> MRTYSSLLEEFATELGLEEIETNELGHGAVTIDKIWVVHLAPINEKELVAFMRAGILTGQSQLYDILRKNLFSPLSGVIRCALDKDDHWLLWSQLNINDT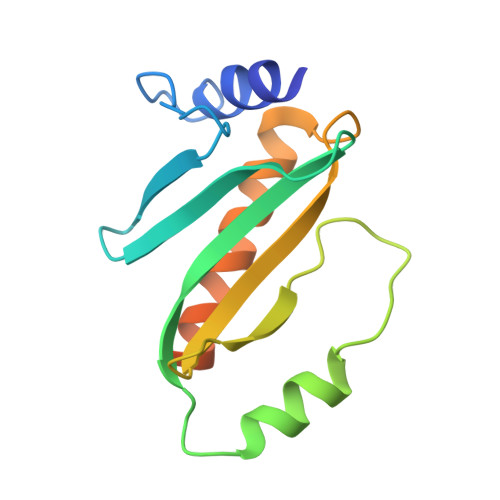SGTQLASVLTSLVDKAVTLSCEPTMKKEEDDHRPSSSH> MADTDTQKADVVVVGSGVAGAIVAHQLAMAGKAVILLEAGPRMPRWEIVERFRNQPDKMDFMAPYPSSPWAPHPEYGPPNDYLILKGEHKFNSQYIRAVGGTTWHWAASAWRFIPNDFKMKSVYGVGRDWPIQYDDLEPYYQRAEEELGVWGPGPEEDLYSPRKQPYPMPPLPLSFNEQTIKTALNNYDPKFHVVTEPVARNSRPYDGRPTCCGNNNCMPICPIGAMYNGIVHVEKAERAGAKLIENAVVYKLETGPDKRIVAALYKDKTGAEHRVEGKYFVLAANGIETPKILLMSANRDFPNGVANSSDMVGRNLMDHPGTGVSFYASEKLWPGRGPQEMTSLIGFRDGPFRATEAAKKIHLSNLSRIDQETQKIFKAGKLMKPDELDAQIRDRSARYVQFDCFHEILPQPENRIVPSKTATDAIGIPRPEITYAIDDYVKRGAAHTREVYATAAKVLGGTDVVFNDEFAPNNHITGSTIMGADARDSVVDKDCRTFDHPNLFISSSATMPTVGTVNVTLTIAALALRMSDTLKKEV;> MGKSTLTFLIAGCLALPGFARAADAADPALVKRGEYLATAGDCMACHTVKGGKPYAGGLGMPVPMLGKIYTSNITPDPDTGIGKWTFEDFERAVRHGVSKNGDNLYPAMPYVSYAKITDDDVRALYAYFMHGVEPVKQAPPKNEIPALLSMRWPLKIWNWLFLKDGPYQPKPSQSAEWNRGAYLVQGLAHCSTCHTPRGIAMQEKSLDETGGSFLAGSVLAGWDGYNITSDPNAGIGSWTQQQLVQYLRTGSVPGVAQAAGPMAEAVEHSFSKMTEADIGAIATYVRTVPAVADSNAKQPRSSWGKPAEDGLKLRGVALASSGIDPARLYLGNCATCHQMQGKGTPDGYYPSLFHNSTVGASNPSNLVQVILNGVQRKIGSEDIGMPAFRYDLNDAQIAALTNYVTAQFGNPAAKVTEQDVAKLRSGGPVPLLVRVRPLMLPGAVVVVLIALLGVAFWWRRRQRTPLANPPQGKAGHH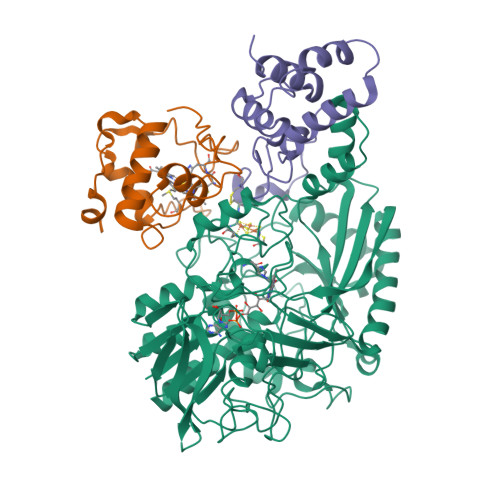HHHH;> DNPGTAPLDTFMTLSESLTGKKGLSRVIGERLLQALQKGSFKTADSLPQLAGALASGSLTPEQESLALTILEAWYLGIVDNVVITYEEALMFGVVSDTLVIRSYCPNKPGFWADKPIERQA> SMKPTKVHIGRLTRNVTKDH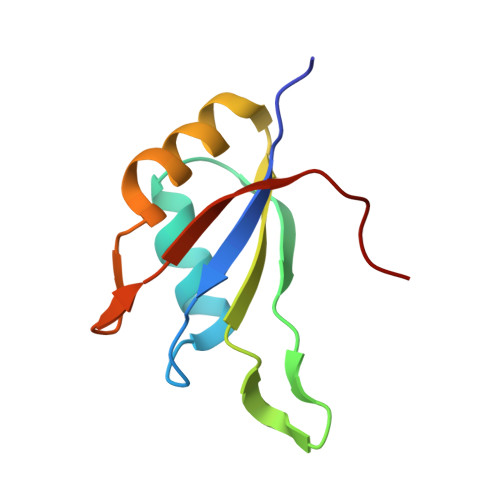IMEIFSTYGKIKMIDMPVERMHPHLSKGYAYVEFENPDEAEKALKHMDGGQIDGQEITATAVLAPWPR>GSSEHLKREHSLIKPYQGVGSSSMPLWDFQGSTILTSQYVRLTPDERSKEGSIWNHQPCFLKDWEMHVHFKVHGTGKKNLHGDGIALWYTRDRLVPGPVFGSKDNFHGLAIFLDTYPNDETTERVFPYISVMVNNGSLSYDHSKDGRWTELAGCTADFRNRDHDTFLAVRYSRGRLTVMTDLE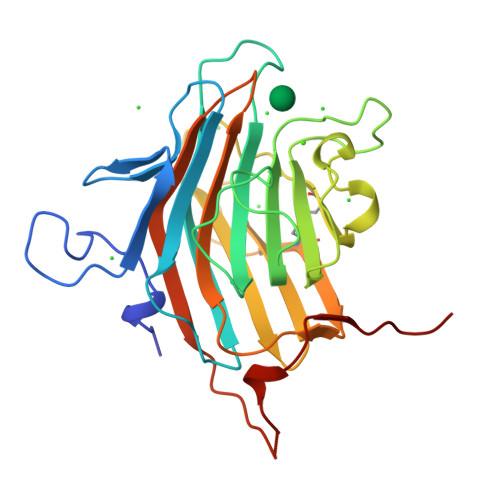DKNEWKNCIDITGVRLPTGYYFGASAGTGDLSDNHDIISMKLFQLMVEHTPDEENIDWTKIEPSVNFLKS[2x]>[2x]PNFSGNWKIIRSENFEELLKVLGVNVMLRKIAVAAASKPAVEIKQEGDTFYIKESTTVRTTEINFKVGEEFE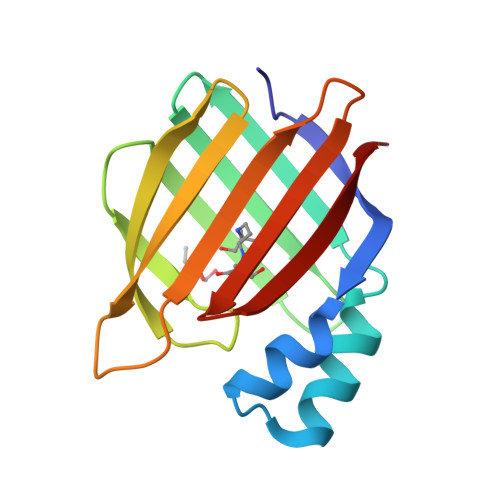EQTVDGRPCKSLVKWESENKMVCEQKLLKGEGPKTSWTLELTNDGELILTMTADDVVCTKVYVRE> GMDTPANKPCIICVAITGSVPTKADNPAVPITVSEQVESTQEAFEAGA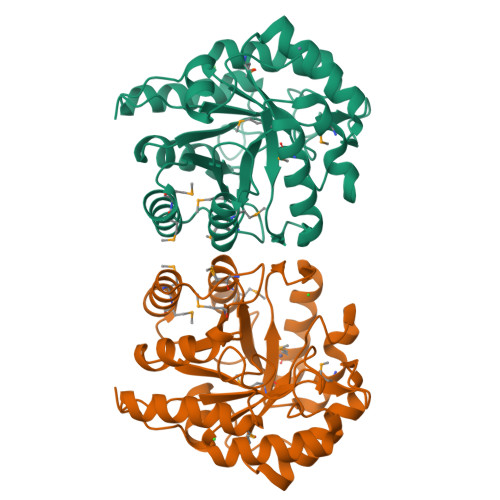AIAHCHVRNDDGTPSSDPDRFARLTEGLHTHCPGMIVQFSTGGRSGAGQARGGMLPLKPDMASLSVGSNNFPSRVYENPPDLVDWLAAQMRSYRVTPEIEAFDLSHILRAIDMHGRGLLYGKLYVQFVMGVKNAMPADREVFDFYVRMMRTRAPQAEWCAAGIGANQLTVNEWAIAAGGHTRTGLEDNIRLDRQTLAPSNAALVRRSVELCDKYQRPVASWQQAREILGLPAAARN3-phenoxy-~{N}-[(~{E})-(5-pyrimidin-2-ylsulfanylfuran-2-yl)methylideneamino]benzamide | C22 H16 N4 O3 S | 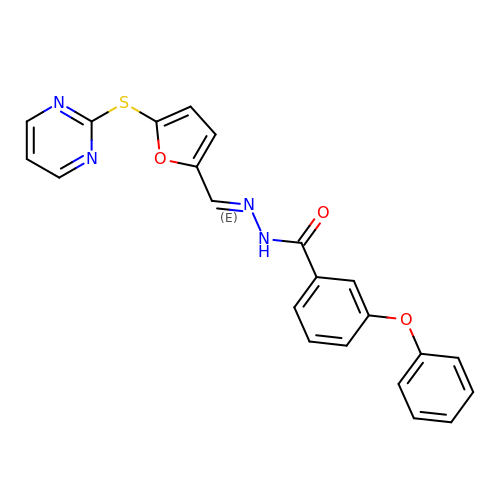ADVBODULINBOOF-MFKUBSTISA-N> MSAEVIHQVEEALDTDEKEMLLFLCRDVAIDVVPPNVRDLLDILRERGKLSVGDLAELLYRVRRFDLLKRILKMDRKAVETHLLRNPHLVSDYRVLMAEIGEDLDKSDVSSLIFLMKDYMGRGKISKEKSFLDLVVELEKLNLVAP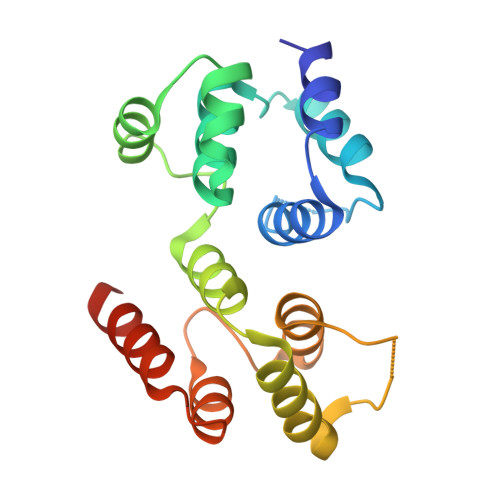DQLDLLEKCLKNIHRIDLKTKIQKYKQSVQGAGTS In class A β-lactamases, a conserved structural element called the omega loop5 constitutes a wall at the active site that shapes the binding cavity. PenL (NCBI reference sequence: YP_439646.1) is highly conserved in pathogenic Burkholderia species, including Burkholderia pseudomallei, Burkholderia mallei, and Burkholderia cenocepacia. PenL has been used as a model in exploring various evolutionary paths to substrate spectrum extension through amino acid substitutions, deletions, and duplications. In this study, we demonstrate the extensive perturbation-absorbing capacity of the omega loop against TR mutations of various sizes, some of which are large enough to include the entire omega loop.

In contrast to the PenL-WT structure, in which every residue could be mapped, PenL-tTR10 and PenL-tTR11 both had a highly disordered region, where the mapping of the residues was not feasible due to high mobility. In PenL-tTR10, two additional residues flanking the first unit on either side were not mapped. In both PenL-tTR10 and PenL-tTR11, it appeared that the α10 helix structure (13 residues: 183–195) downstream of (in the case of PenL-tTR10) or overlapping (in the case of PenL-tTR11) the tTR required the second repeat unit of the tTR, instead of the first unit, to be in place in the protein backbone. In the PenL-tTR structures, perturbations in the omega loop resulted in the dislocation of a number of nearby residues, along with the disorganization of the α-helix in the omega loop (Glu166-Asn170), which most notably led to the breakage of a salt bridge that is normally present between Thr167 and Arg104 and tightly packs the active-site cavity. In PenL-tTR10, the side chain of Asn170 exhibited a particularly large movement of 9.63 Å, causing it to swing 180° from the active site cavity. Furthermore, the side chain of Asp240 was rotated approximately 90°, moving away from the active site by 3.21 Å in PenL-tTR10 and by 2.89 Å in PenL-tTR11. The side chain of Tyr105, which is known to be involved in substrate recognition and the stabilization of the enzyme-substrate complex, was flipped and moved away from the active site by 1.17 Å in tTR10 and by 1.00 Å in tTR11. The volume of the active site in PenL-tTR10 was 274.9 Å3, as measured with CASTp29. This is much larger than that of PenL-WT, which was 182.3 Å3, demonstrating the extreme expansion of the active sites in the mutant enzyme. In PenL-tTR10, the interaction between W1 and the general base Glu166 remained, although the geometry was altered.

>[2x]GSHMRNVAAEQQLRELESTFDGRLGFVALDTATGARIAHRADERFPFCSTFKTMLSAAVLARSAGDAALLQRRIPYAKRDLVRYSPITEKHVGAGMTVAELCAATLQYSDNTAANLLIALLGGPQAVTAYARSIGDATFRLDRRETELNTAIPGDERDTTTIPGDERDTTTPAAMAASVRRLLVGDALGTAQRAQLNAWMLGNKTGDARIRAGVPAGWRVADKTGTGDYGTGNDIGVAYPPDRAPIVFVVYTTMRSRNAQARDDVIASAARIAARAFV>GHMQEGEQLMSYINRDLENLQERIIARANEWLAAEQKSAKSKETEQLAAMVHDPSGVEFTMRFVDRVARPQDNQVAARELTKLTDTELPGFIGPIDRALVNTGAKMAKFVPNFIMPAARTRLRQMVSHLVLDAEGKALNKLLDESKAKGYRLNVNLLGEAVLGDGEANNRLTRTMELLKNPRVDYVSIKATSVVAQLNPWDIDGNTELLKERLRPLYRLALQRSPHPFINLDMEEYKDLHVTIRLFEELLMEEEFLGLEAGIVLQAYLPDSFQALQQLADFAKRRAAAGGAKIKIRLVKGANLSMEKVDAELHGWYPAPYATKEEVDANFLRMMDYILRPEHENVRVGIASHNLFSVASAYELSVERGVETQLDVEMLQGMAPAQAEAVRQAVGTVILYTPVVHAEDFDVAVSYLVRRLEENGAPENFLYALFGGDLTEQEARFRESVAQRWKVAEDSRRLSTPETFNASDSDPALLSTLEWARTLEDPQPKWRLITDVEEVDKTVAGLLKSPRLDIAERTALLQRAADELENIRQDLLGVMTHEAGKTIAEADPEVSEAIDFARYYARCANALNTPGHSKFTPHNLVVVASPWNFPVAIPLGGVFASLAAGAK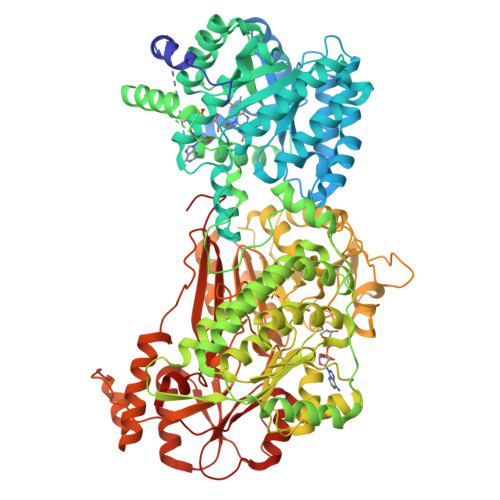AILKPAPEVRRCAEVALTALRKAGIGEDLVQLMHTDEADAGRRLMSHPDVDAIILTGASETASLFRGWKPEMNIHAETSGKNAIIVTPSADPDLAVADVYKSAFGHAGQKCSAASLVILVGDVGRFTDQLIDATRTLRVGYGHELSTTMNGLISPPGEKLHRGLTTLETGESWLVKPEKLNDEGTLWSPGIRDNVRPGSWFHTHECFGPVLGIMHAESLEQAIEWQNSTGFGLTGGIHSLDEDEVELWKEKVEVGNAYINRGITGAIVQRQPFGGWKNSSVGVGAKAGGPNYVAQLGTWEDIESDVPSVSLPPAYRELANTEFLKRAAALDEIAWRTEFGVEQDFTGLRCESNVFRYRPLETLYVVGDDEEQFNRLKLAALRTGTELRKLETHEWFPPHSRIRAIGDAPVPTTIYEWAALNGSVVIDGPVLADGRRELLHFLKEQAVSTTNHRFGYIKEETS[4x]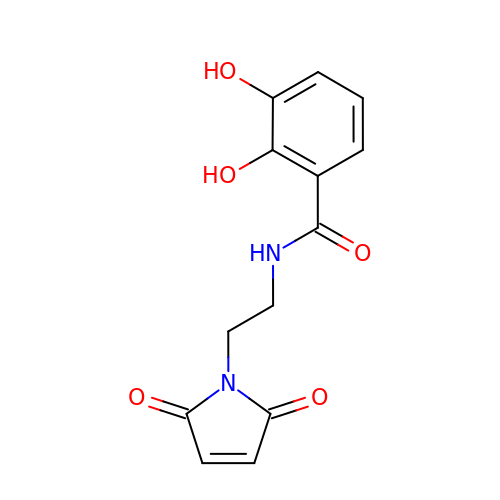N-[2-[2,5-bis(oxidanylidene)pyrrol-1-yl]ethyl]-2,3-bis(oxidanyl)benzamide | C13 H12 N2 O5 | BABSFPLAEBUXOA-UHFFFAOYSA-N AppA, the Escherichia coli periplasmic phytase of clade 2 of the histidine phosphatase (HP2) family, has been well-characterized and successfully engineered for use as an animal feed supplement. The E. Coli periplasmic phytase, AppA, is a 1D-6-phytase (EC 3.1.3.2) and initial hydrolysis preferentially liberates the phosphate at the 1D-6-position on the inositol ring. HP2Ps catalyse the hydrolysis of phytate via an obligatory phosphohistidine intermediate. The catalytic proton donor is found in a second, short, conserved motif with sequence HD positioned such that the aspartic acid residue functions as the consensus proton donor in the catalytic mechanism.

Notably, KM was 5-fold lower than wild type for the proton donor-less AppA-HAT variant and the MINPP-like AppA-HAE double mutant. The low turnover numbers (kcat) for these hydrolysis-compromised variants (only ~0.1% of that seen for the wild-type enzyme) suggests that breakdown of the phosphohistidine intermediate is rate limiting. Of the remaining variants, AppA-HAE showed a marginally increased production of InsP5 [1/3-OH] (22% of the total InsP5), while AppA-HET proved to be more catalytically flexible producing almost equal amounts of InsP5 [1/3-OH] and InsP5 [4/6-OH]. At residue position 305, the T305E substitution found in the AppA-HDE and -HAE variants results in sidechain χ1 angles of 46° and 65°, respectively, for the glutamate residue. The residue therefore adopts the g− conformation rather than the preferred g+ conformation for glutamate observed in α-helical environments, which is seen in bacterial MINPPs for which crystal structures are available. The g+ rotamer is required for the carboxyl group of this residue to approach the phosphomonoester bridging oxygen in the specificity pocket A to allow it to function as a proton donor in catalysis. Thus, in the AppA-HAE and -HDE variants the E305 sidechain points away from the substrate and towards the active site cavity. The inability of E305 to participate in catalysis is reflected in the similarity of the kinetic parameters for AppA-HAE to those of the proton donor-less AppA-HAT variant and low turnover number for hydrolysis of phytate. AppA-HDE has slightly enlarged pockets A and B due to the loss of the side-chain methyl group of T305, whereas the double mutant AppA-HAE has larger pockets A and B with an overall change in polarity. For both variants, pocket F decreases in size and its polarity increases by virtue of introduction of the larger sidechain of and carboxyl group of glutamate.

> GPQSEPELKLESVVIVSRHGVRAPTKATQLMQDVTPDAWPTWPVKLGWLTPRGGELIAYLGHYQRQRLVADGLLAKKGCPQSGQVAIIADVDERTRKTGEAFAAGLAPDCAITVHTQADTSSPDPLFNPLKTGVCQLDNANVTDAILSRAGGSIADFTGHRQTAFRELERVLNFPQSNLCLKREKQDESCSLTQALPSELKVSADNVSLTGAVSLASMLTEIFLLQQAQGMPEPGWGRITDSHQWNTLLSLHNAQFYLLQRTPEVARSRATPLLDLIKTALTPHPPQKQAYGVTLPTSVLFIAGHAENLANLGGALELNWTLPGQPDNTPPGGELVFERWRRLSDNSQWIQVSLVFQTLQQMRDKTPLSLNTPPGEVKLTLAGCEERNAQGMCSLAGFTQIVNEARIPACSL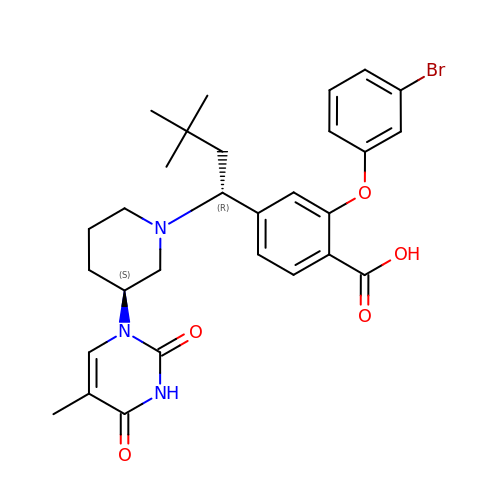2-(3-bromophenoxy)-4-{(1R)-3,3-dimethyl-1-[(3S)-3-(5-methyl-2,4-dioxo-3,4-dihydropyrimidin-1(2H)-yl)piperidin-1-yl]butyl}benzoic acid | C29 H34 Br N3 O5 | SXYGLXXKMZTVNB-XUZZJYLKSA-N Rhinoviruses (RVs) are the main cause of the common cold. Belonging to the large family Picornaviridae, the typical architecture of RVs comprises a ~ 30 nm diameter capsid enclosing a ss(+) RNA genome of about 7200 bases. The building blocks are four capsid proteins (VPs) present as 60 copies each and arranged on a pseudo T = 3 lattice. After the first 3Dstructures of RV-B146 as well as of the closely related poliovirus type 17 had been solved, high-resolution X-ray and cryo-electron microscopy (cryo-EM) structures of numerous RV types and of closely related members of the Enterovirus genus became available and have been used for the design of capsid-binding compounds. These drug candidates attach inside a hydrophobic pocket mainly contributed by amino acid residues of VP1 and displace a natural pocket factor—in most cases a myristate—stabilizing the viral shell against structural changes required for release of the viral RNA genome into the host cell’s cytosol for infection.

During 2D classification of the extracted particle images we also noted that about 20% of the particles represented empty capsids. Following the infection and virus purification protocol, we usually found empty particles in the range of a low two-digit percentage of total viral particles. For completeness, we also analyzed the structure of the reconstructed empty capsid (the B particle); it also exhibits an empty and collapsed hydrophobic pocket missing the myristate; similarly to the native empty structure, residue VP1-Met222 reaches into the pocket. This agrees with previously published structural data of uncoated particles. Finally, based upon our structural data we conclude that incubation of RV-A89 with DMSO elutes the myristate from the hydrophobic pocket and renders the conformation of the pocket more like the pocket of the uncoated virion.

> TRDETSIESFLGRSGCIAMIEFNTSSDKTEHDKIGKGFKTWKVSLQEMAQIRRKYELFTYTRFDSEITIVTAAAAQGNDSGHIVLQFMYVPPGAPVPEKRDDYTWQSGTNASVFWQEGQPYPRFTIPFMSIASAYYMFYDGYDGDSAASKYGSVVTNDMGTICVRIVTSNQKHDSNIVCRIYHKAKHIKAWCPRPPRAVAYQHTHSTNYIP;> IQITRGDSTITSQDTANAVVAYGVWPSYLTPDDATAIDKPTQPDTSSNRFYTLDSRSWTSASSGWWWKLPDALKNMGIFGENMFYHFLGRSGYTIHVQCNSSKFHQGLLIVAAIPEHQLASATSGNVSVGYNHTHPGEQGREVVPSRTSSDNKRPSDDSWLNFDGTLLGNLPIYPHQYINLRTNNSATLILPYVNAVPMDSMLRHNNWSLVIIPICPLQVQPGGTQSIPITVSISPMFSEFSGPRS;> PVMLTPGSGQFLTTDDTQSPSAFPYFHPTKEIFIPGQVRNLIEMCQVDTLIPVNNTQENVRSVNMYTVDLRTQVDLAKEVFSIPVDIASQPLATTLIGELASYYTHWTGSLRFSFMFCGSASSTLKLLIAYTPPGVGKPKSRREAMLGTHLVWDVGLQSTASLVVPWVSASHFRFTTPDTYSSAGYITCWYQTNFVVPDSTPDNAKMVCMVSACKDFCLRLARDTNLHT Hp0323 (NucT) encodes a nuclease from Helicobacter pylori belonging to the endonuclease PLD sub-family. So far, NucT has been implicated both in the process of natural transformation and in the purine salvage pathway. The family is defined by the “HxK(x)4D(x)6GSxN” sequence signature where the histidine is proposed to act in all PLD enzymes as a nucleophile in a phosphodiester bond cleavage. In summary, these results show that NucT has an endonuclease activity with a strong preference for single-stranded DNA (or RNA) substrates, over double-stranded ones.

Twelve identical copies of NucT are present in the asymmetric unit of the crystal (rmsd ranged from 0,7413 to 0,8494 Å taken monomer A to the 11 others), forming 6 identical dimers (rmsd from 0,5647 to 0,6868 Å) with a 2-fold rotational symmetry axis. The active site of NucT and of its homologues is carried by the loops that link its seven-stranded β-sheet, itself surrounded on one side by 5 α-helices and on the other side by one long α-helix. The HxK(x)4D(x)6GSxN signature of NucT is perfectly superimposable with the catalytic centers of Nuc and Zucchini. NucT formed dimers in the crystal, a feature in common with all the PLD superfamily members described so far. The active site, twinned by the dimerization, is nested in the hollow of its dimer interface, surrounded by two small helices and long loops (orange in Fig 5A). The substrate specificity of NucT (i.e. single-stranded vs double-stranded nucleic acids) could then be determined by the restriction of the accessibility of the active site due to the two negative patches. However, a major difference between NucT and Nuc or Zucchini resides in the presence of an extra loop present exclusively in the NucT structure. While the short loops present in Nuc and Zuc are acidic (pI 4.2 and 5.7 respectively), the extra loop in NucT carries a strong positive charge, with a local pI close to 10. Thus, the NucT loop might contribute to attract the DNA into the electrostatic groove of the dimer, resulting in the higher affinity for the ssDNA when compared to Zuc.

>GISEFKNSLFVLPYEQRDALNSLISGISSARESVKIAIYSFTHRDIARAIKSVASRGIKVQIIYDYESNHNNKQSTIGYLDKYPNTKVCLLKGLKAKNGNYYGIMNQKVAIIDDKIVFLGSANWSKNAFENNYEVLLKTDDTETILKAKSYYQKMLESCVGF[12x]HVEM is a TNF (tumor necrosis factor) receptor contributing to a broad range of immune functions involving diverse cell types. It interacts with a TNF ligand, LIGHT, and immunoglobulin (Ig) superfamily members BTLA and CD160. HVEM engages in bidirectional signaling, serving not only as a receptor but also as a ligand for IgSF receptor signaling. To dissect the molecular basis for multiple functions, we determined crystal structures that reveal the distinct HVEM surfaces that engage LIGHT or BTLA/CD160, including the human HVEM–LIGHT–CD160 ternary complex, with HVEM interacting simultaneously with both binding partners.

Here, we report the structures of human orthologues of members this network, including the ternary hHVEM–hLIGHT–hCD160 and binary hHVEM–hLIGHT complexes; we also report the structure of mHVEM in isolation. Based on structural and sequence alignments between hHVEM and mHVEM, the solvent-accessible mHVEM residues close to the putative binding interfaces were mutated to dissect the interaction network and enable in vivo HVEM functional studies. A total of 52 mHVEM surface residues within or close to the likely ligand-binding interfaces were individually mutated to different amino acids to probe the effect on ligand binding and to identify variants with selective ligand recognition. For example, alteration of mHVEM G72 or V74 to aspartic acid attenuated binding to both mBTLA and mCD160, but not binding to mLIGHT; the mHVEM R43D, M56D, or A76D mutations decreased binding to mCD160, but not mBTLA and mLIGHT; and the mHVEM H86D, L90A, L94A, and L94D mutations compromised the interaction with mLIGHT, but not mBTLA or mCD160. The mHVEM G72R-V74A double mutation exhibited no binding to mBTLA or mCD160, while it retained WT binding to mLIGHT in our cell–cell and cell–protein interaction system. The mHVEM H86D-L90A double mutation showed no binding to mLIGHT and WT binding to mBTLA and mCD160.

> QPSCRQEEFLVGDECCPMCNPGYHVKQVCSEHTGTVCAPCPPQTYTAHANGLSKCLPCGVCDPDMGLLTWQECSSWKDTVCRCIPGYFCENQDGSHCSTCLQHTTGHHHHHH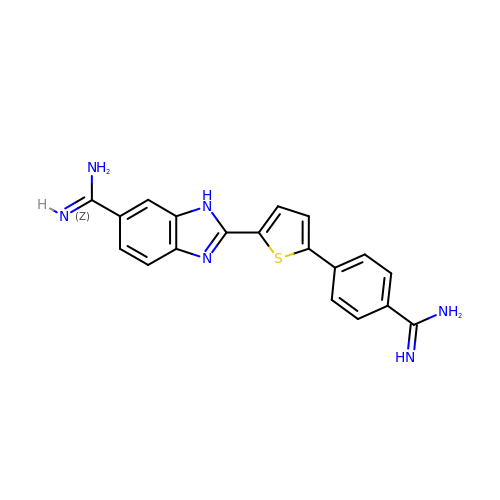2-(5-{4-[AMINO(IMINO)METHYL]PHENYL}-2-THIENYL)-1H-BENZIMIDAZOLE-6- CARBOXIMIDAMIDE DIHYDROCHLORIDE | C19 H16 N6 S | MSQVFIHMHRAMOC-UHFFFAOYSA-N>MLGVIADDFTGASDIASFLVENGLSTVQMNGVPTQSLNSKVDAIVISLKSRSNPVNEAIEQSLRAYQWLKENGCTQFYFKYCSTFDSTAKGNIGPVTDALLDELNEDFTVITPALPVNGRTIFNGYLFVGDVLLSESGMKNHPITPMVDANLMRLMDAQAKGKTGLVAYADVIKGASRVQECFAELKAQGYRYAVVDAVDNSQLEVLAEAVADFKLVTGGSGLGAYMAARLSGGKKGTNAFTPTKGKTVVLSGSCSVMTNKQVEKYREKAPHFQLDVEQAIHNENYIEQLYQWVIANLDSEFAPMVYATVPPDALKAIQHQFGVDQASHAIENTFAKLAAKLKQYGVTNFITAGGETSSIVVQELGFTGFHIGKQIAPGVPWLKAVEEDIFLALKSGNFGK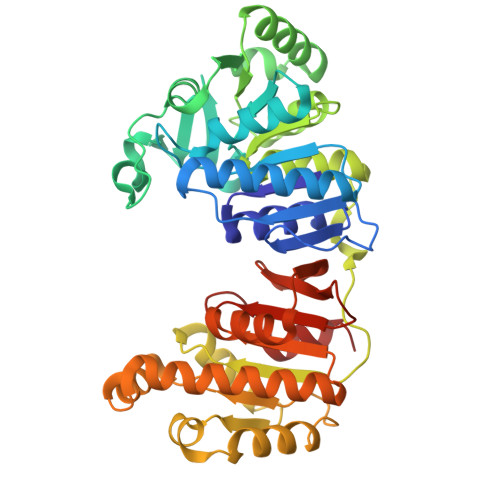EDFFEYAQGMFL[2x]3-PHENYLPROPYLAMINE 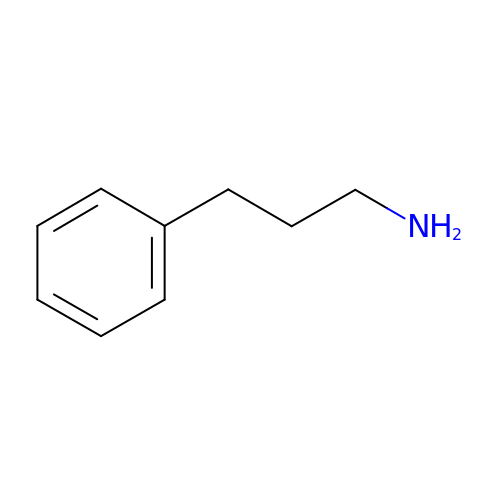| C9 H13 N | LYUQWQRTDLVQGA-UHFFFAOYSA-N>MGSHHHHHHGRSAAGTMANLDKMLNTTVTEVRKFLQADRVCVFKFEEDYSGTVSHEAVDDRWISILKTQVQDRYFMETRGEEYVHGRYQAIADIYTANLVECYRDLLIEFQVRAILAVPILQGKKLWGLLVAHQLAG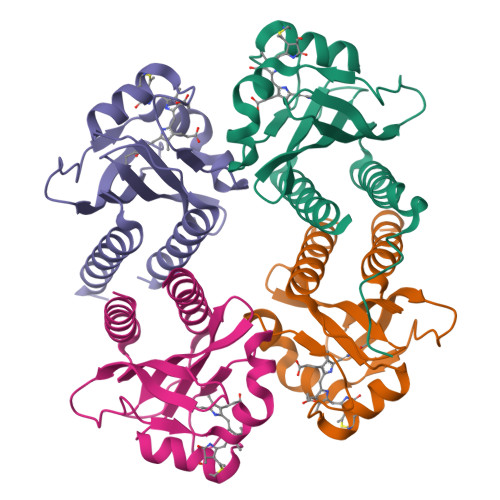PREWQTWEIDFLKQQAVVMGIAIQQS[4x]>[2x]GSHMHGTAFVVKLRG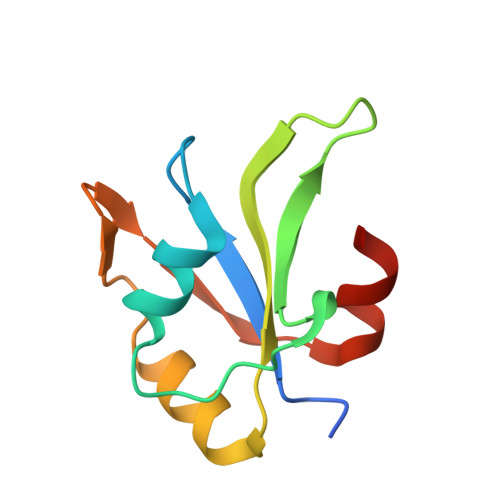LPYAVTEQQIEEFFSGLDIKTDREGILFVMDRRGRATGEAFVQFESQDDTEQALGRNREKIGHRYIEIFRSSIAEMKRATGA> GPLGSPEFPHPLQDSWSYYLFQFRKALDWDECLEKVATFSTIEDFWSVLTHTVRPREITYGKDLYMFKSDIMPKWEDPKNENGGRWLINVTARQDVDF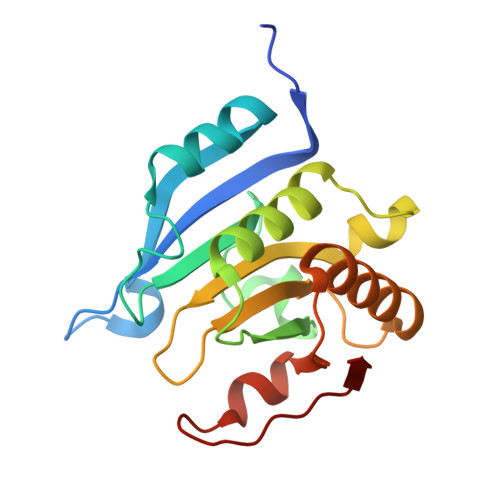LWDELLMLLIGSDWDTDEEDRQICGAVFQPRSRGSKLSVWLTSDNEEETILSIGRRIKERLELEDTIYFQPVSDQRSQTRGSDICTGKYEI>MPDTAINPRDPVFVSYRHSDGIALAAELTWLLRAAGIPVWRDVDDLPPGDTDARLQQAIDEGISGAVIIITPQIADSRVVREVEAPRLLRLHRSSPQFALGIVNAIQTSTGVVDYDAPDRVLGMERPELRSVDQKSASRLGLVTMARQMLWHRIAAIRPLLSASGGELRLSLQTRNTPQVYDRTDADLDIRIRPSAHEKLPSAHGLEDFAETAQFLPDAVTRAGANGVRIEGGAHLSVSIAIGAAIPSTRVGPMTVVDGRGVHWVSSTEPQLPDEPRLRIVRESTIPSTAPAPGRPDVAAYIDLQHPRSDAAFDNYLT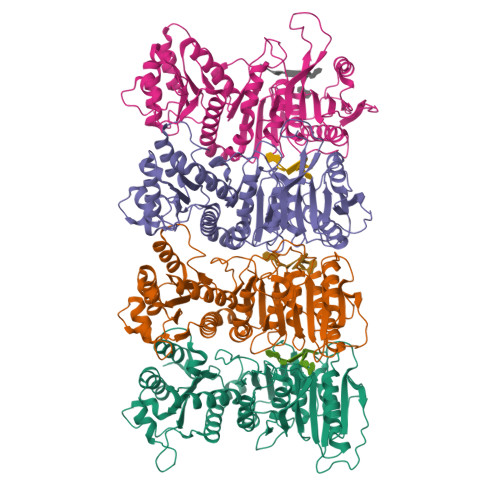EHAAELVAWQHLAPTRTGLLDAADGGTIAAEAVAHIRELSMTNGNAVVHLMVRGPFGLAVLIGRLTNTLRVVAYEWTDSDAPDGTFMPPRYEPIVQLRASTPAGVIERVIVADAE[4x]>[2x]DLKWEFPRENLEFGKVLGSGAFGKVMNATAYGISKTGVSIQVAVKMLKEKADSSEREALMSELKMMTQLGSHENIVNLLGACTLSGPIYLIFEYCCYGDLLNYLRSKREKFSEDEIEYENQKRLEEEEDLNVLTFEDLLCFAYQVAKGMEFLEFKSCVHRDLAARNVLVTHG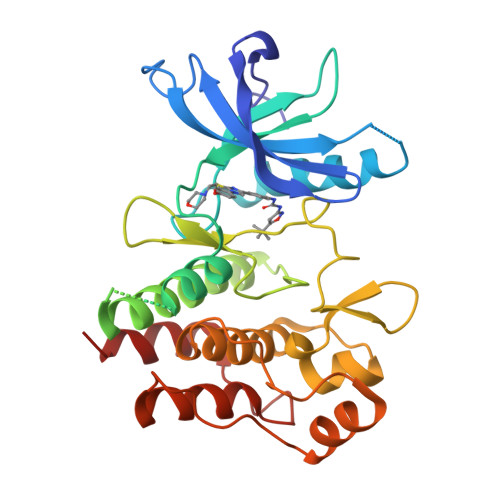KVVKICDFGLARDIMSDSNYVVRGNARLPVKWMAPESLFEGIYTIKSDVWSYGILLWEIFSLGVNPYPGIPVDANFYKLIQNGFKMDQPFYATEEIYIIMQSCWAFDSRKRPSFPNLTSFLGCQL Here, it is reported that multiple zinc ions can easily be charged onto the surface of proteins with no intrinsic zinc-binding site by using zinc-containing solutions. Here, we show that the surface of proteins can be charged with zinc ions and that the anomalous signals from these zinc ions can be used for structure determination of proteins. In conclusion, we demonstrated that protein crystals grown in the presence of zinc ions or soaked in a zinc-containing solution are easily charged with multiple zinc ions on the protein surface and that they are suitable for zinc SAD/MAD phasing. Considering the high phasing effectiveness and multiple zinc-binding sites, we believe that zinc derivatization of the protein surface is a largely unnoticed but promising method for phase determination of protein crystals.

Recently, we obtained crystals of TON_0340 in a precipitant solution containing zinc acetate. The TON_0340 crystals, which contained six molecules per asymmetric unit, belonged to the tetragonal space group P43212, with unit-cell parameters a = b = 107.44, c = 355.03 Å. Additionally, three zinc ions bound to a cluster of six acidic residues were located in a putative active-site cleft.

>MIAHLINTDIGNRGVLKVYLDYRRKNFNFLHNSTKMFLDNLERVLIVTGFPIPPMMVAETDGPPGALAIYRAVEMLGGKAEILTYSEVEKALEPFGVSLARTPEPEDYSLIISVETPGRAADGRYYSMSALEIKRDPLDGIFLKARALGIPTIGVGDGGNEIGMGKIRELVVGHVPHGEKIASVVETDELIVSAVSNWGAYGLVAQASIEVGRNLLEGWDERRVIEAISSAGLIDGVSKTLAPSVDGIRLMVHEGIVELLKAVVDEAIL[6x]2-[(3S)-piperidin-3-yl]-1,3-benzoxazole | C12 H14 N2 O | 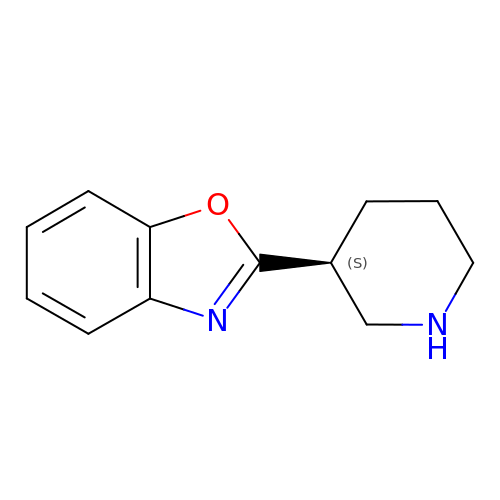MNJITFGKRQIUJN-VIFPVBQESA-N4-[3-(TRIFLUOROMETHYL)DIAZIRIDIN-3-YL]-L-PHENYLALANINE | C11 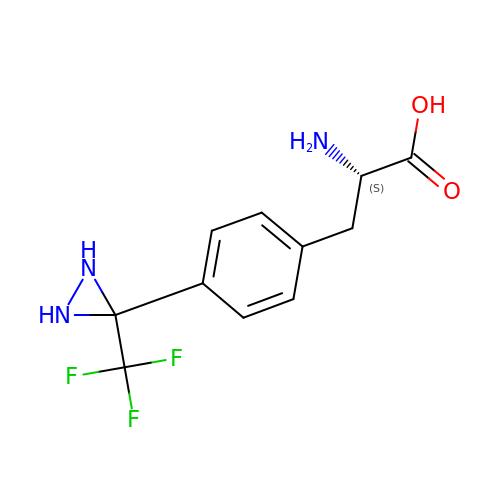H12 F3 N3 O2 | XCRAOXMHVJUSSJ-QMMMGPOBSA-N> GSHMARGKLKAPKWPILKNLELLQAQNYSRNIKTFPYKELNKSMYYDKWVCMCRCEDGALHFTQLKDSKTITTITTPNPRTGGEHPAIISRGPCNRLLLLYPGNQITILDSKTNKVLREIEVDSANEIIYMYGHNEVNTEYFIWADNRGTIGFQSYEDDSQYIVHSAKSDVEYSSGVLHKDSLLLALYSPDGILDVYNLSSPDQASSRFPVDEEAKIKEVKFADNGYWMVVECDQTVVCFDLRKDVGTLAYPTYTIPEFKTGTVTYDIDDSGKNMIAYSNESNSLTIYKFDKKTKNWTKDEESALCLQSDTADFTDMDVVCGDGGIA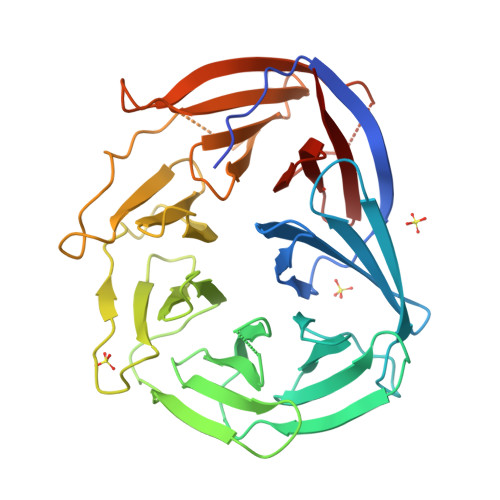AILKTNDSFNIVALTP> SNAME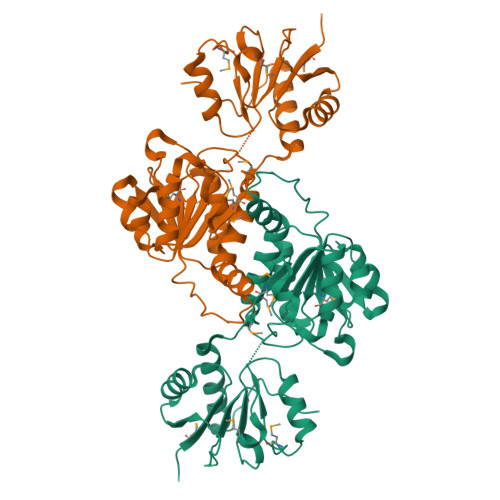IIFYHPTFNAAWWVNALEKALPHARVREWKVGDNNPADYALVWQPPVEMLAGRRLKAVFVLGAGVDAILSKLNAHPEMLDASIPLFRLEDTGMGLQMQEYAVSQVLHWFRRFDDYQALKNQALWKPLPEYTREEFSVGIMGAGVLGAKVAESLQAWGFPLRCWSRSRKSWPGVESYVGREELRAFLNQTRVLINLLPNTAQTVGIINSELLDQLPDGAYVLNLARGVHVQEADLLAALDSGKLKGAMLDVFSQEPLPQESPLWRHPRVAMTPHIAAVTRPAEAIDYISRTITQLEKGEPVTGQVDRARGY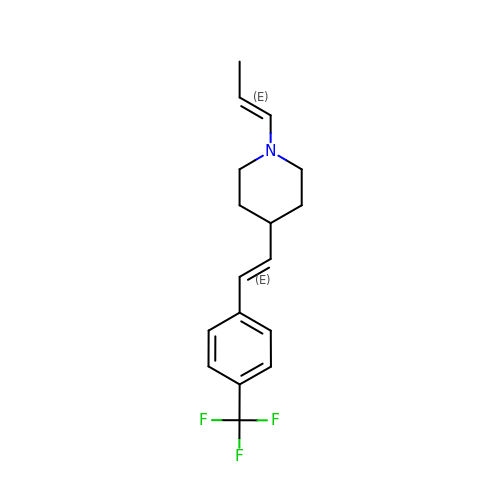1-[(~{E})-prop-1-enyl]-4-[(~{E})-2-[4-(trifluoromethyl)phenyl]ethenyl]piperidine | C17 H20 F3 N | ONJVYKXNJUTMAU-FRKQTSRXSA-N5-[3-(aminomethyl)phenyl]-~{N}-[(2~{S},3~{S},4~{R},5~{S},6~{S})-6-methyl-3,4,5-tris(oxidanyl)oxan-2-yl]furan-2-carboxamide 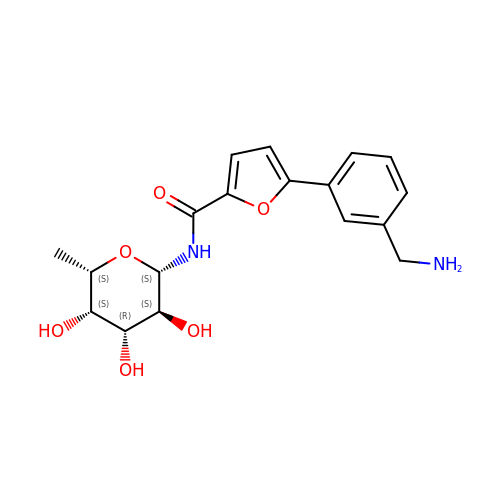| C18 H22 N2 O6 | NOVNWDXRBIJEJE-GUJIERIFSA-N(1S,2S,3S,4R,5R)-4-(morpholin-4-yl)-2-[(quinolin-3-ylmethyl)amino]-6,8-dioxabicyclo[3.2.1]octan-3-ol 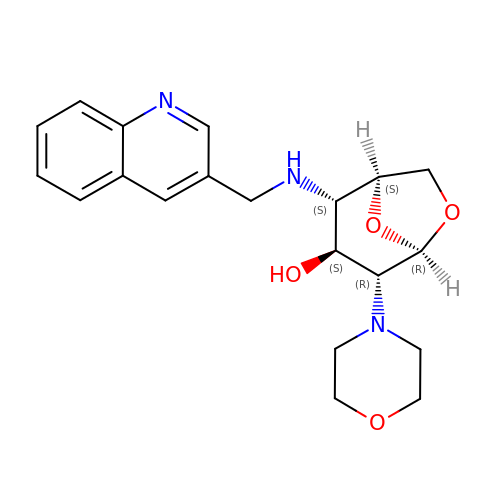| C20 H25 N3 O4 | BOMGHVJKULNWEW-LTFPLMDUSA-N>AAAAAACUUACUAUUAUAUUUGUAACAAAUUUUAUACAUAAGAUAAAUUCGUAUGUAUAGCCGUUCUGCUCGAAACGGUAUAGCACCGUAAUGGUGGUAUUAUGAAUU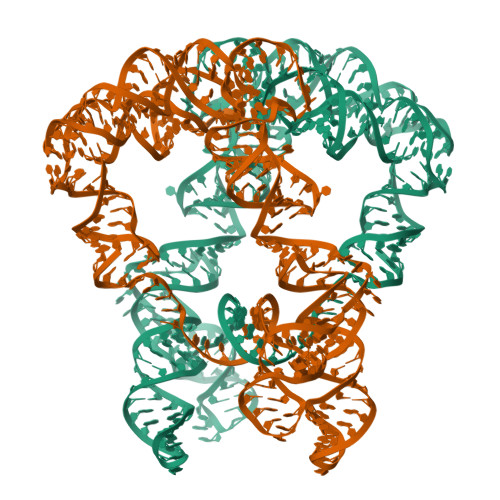GUAGCAAGGUGCGAGGCUACCUUUAAAAGUCUUGGAGGUGCUCUGAGUGGGUACUUUAUUAGGGUUAUAAUUUAGAAAGUAAGCUAAAACUCUAGGUGUUGGGCAGGGCUAACACUGGCAUAUAAUUAAAUAUGCGAUAAAGUAAGU[2x]> GPMAETLEFNDVYQEVKGSMNDGRLRLSRQGIIFKNSKTGKVDNIQAGELTEGIW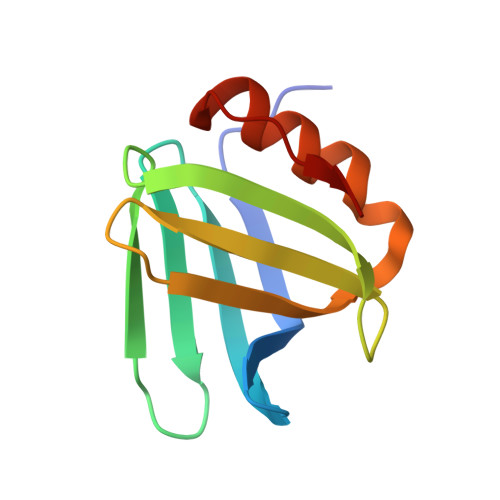RRVALGHGLKLLTKNGHVYKYDGFRESEFEKLSDFFKTHYRLELMEK>[2x]GHMAEKAR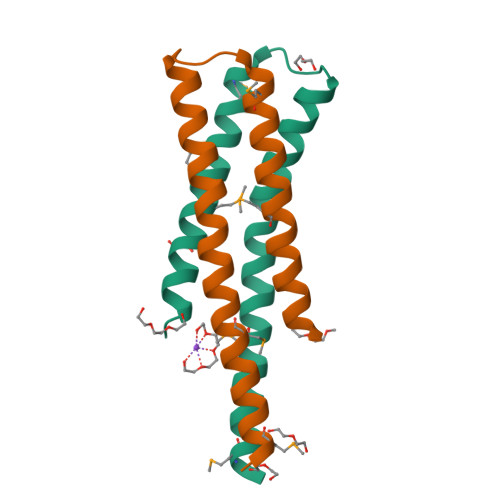DSEDRMRQFITDASHELRTPLTTIRGFAELYRQGAARDVGMLLSRIESEASRMGLLVDDLLLLAKL>[2x]SMRPALYFCGSIRGGREDRTLYERIVSRLRRFGTVLTEHVAAAELG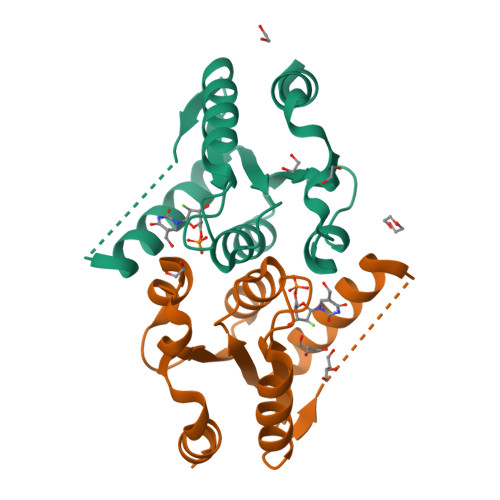ARGEEAAGGDRLIHEQDLEWLQQADVVVAEVTQPSLGVGYELGRAVAFNKRILCLFRPQSGRVLSAMIRGAADGSRFQVWDYEEGEVEALLDRYFEADP> AAF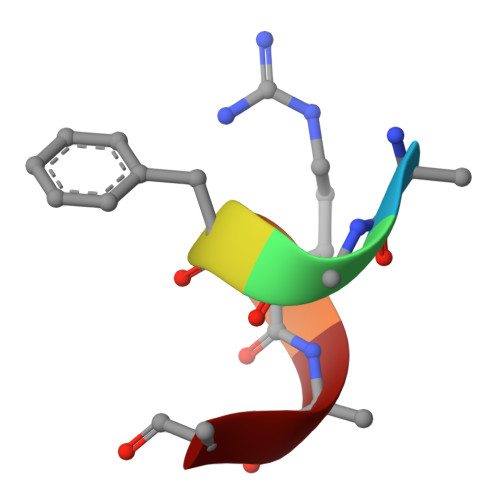RAA> GPGSMRLGRIASPDGVAFVSIEGEDGREESAIAREIAEHPFGTPTFTGRQWPLADVRLLAPILASKV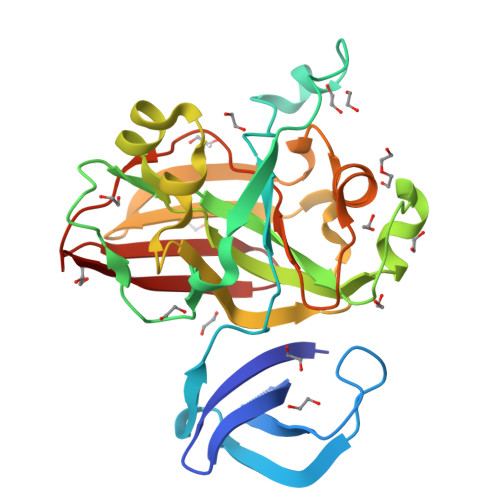VAMGKNYAAHAAEMGGDPPESPVIFIKPNTSIIGPGLPIQLPPSATEVHHEGELAIVIGRPCKDVPAARAAENILGYTIGNDVSARDHQRADGQWTRAKGHDTFCPLGPWIVTDLDPADLEIRTEVNGQVRQRSRTSLLLHDVGAIVEWVSAVMTLLPGDVILTGTPEGVGPIVDGDTVSVTIEGIGTLSNPVVRKAK>[12x]MAQNLKDLAGRLPAGPRGMGTALKLLLGAGAVAYGVRESVFTVEGGHRAIFFNRIGGVQQDTILAEGLHFRIPWFQYPIIYDIRARPRKISSPTGSKDLQMVNISLRVLSRPNAQELPSMYQRLGLDYEERVLPSIVNEVLKSVVAKFNASQLITQRAQVSLLIRRELTERAKDFSLILDDVAITELSFSREYTAAVEAKQVAQQEAQRAQFLVEKAKQEQRQKIVQAEGEAEAAKMLGEALSKNPGYIKLRKIRAAQNISKTIATSQNRIYLTADNLVLNLQDESFTRGSDSLIKGKK;>MAAKVFESIGKFGLALAVAGGVVNSALYNVDAGHRAVIFDRFRGVQDIVVGEGTHFLIPWVQKPIIFDCRSRPRNVPVITGSKDLQNVNITLRILFRPVASQLPRIFTSIGEDYDERVLPSITTEILKSVVARFDAGELITQRELVSRQVSDDLTERAATFGLILDDVSLTHLTFGKEFTEAVEAKQVAQQEAERARFVVEKAEQQKKAAIISAEGDSKAAELIANSLATAGDGLIELRKLEAAEDIAYQLSRSRNITYLPAGQSVLLQLPQ[12x]

Prohibitin complexes are dome-like structures consisting of prohibitin -1 and -2 heterodimers that assemble in the IMS via their N-terminal transmembrane helix. Prohibitin-1 and -2 (PHB1 and PHB2) are members of the Stomatin/prohibitin/flotillin/HflKC (SPFH) protein family. Among other proposed functions, the prohibitin complex supports cristae architecture and negatively regulates the activity of the matrix-resident AAA protease (m-AAA), which cleaves numerous matrix and IM proteins. Three-dimensional (3D) subclassification of the subtomogram averages revealed two distinct conformational states of the prohibitin complex present in untreated and OA-treated cells, both of which resolved to approximately 20 Å.

We termed these two conformational states “open” and “closed” on the basis of detectable protein density for the dimeric membrane-anchoring domains of the prohibitin complex. Density for all 12 heterodimer pairs was visible in our initial subtomogram average, allowing us to model a fully enclosed dome complex. Finally, the top of the dome is assembled by tight packing of the C-terminal helix C-α2, leaving a central pore that is formed from the disordered C-terminus that forms a beta strand complementation with adjacent subunits. Prohibitin 2 contains an additional C-α3 that sticks up above the dome cap. This fully assembled closed prohibitin dome is approximately 20 nm in diameter and rises 10 nm above the membrane. We refer henceforward to the fully assembled state as the closed conformation. The closed conformation manifests additional density extending 3 nm on the matrix side of the IMM, while the open complex is associated with minimal matrix density. An additional unmodeled density occupying 180 nm3 was present on the matrix side of the membrane which cannot be accounted for by prohibitin itself. There is insufficient unmodeled mass in prohibitin 1 and 2 to account for this density, which therefore most likely reflects ordered portions of prohibitin-associated proteins or alterations to bilayer organization. Quantification of the two populations of complexes revealed a statistically significant shift from 75 open to 56% open after depolarization, indicating that the prohibitin complex is basally in a dynamic assembly of states and that depolarization drives the complex toward closure. Under depolarization, prohibitin shifts to the closed “inactive” state, which could, in principle, reduce the degradative capacity of m-AAA with respect to integral membrane proteins of cristae.> MSEKHPGPLVVEGKLTDAERMKHESNYLRGTIAEDLNDGLTGGFKGDNFLLIRFHGMYQQDDRDIRAERAEQKLEPRHAMLLRCRLPGGVITTKQWQAIDKFAGENTIYGSIRLTNRQTFQFHGILKKNVKPVHQMLHSVGLDALATANDMNRNVLCTSNPYESQLHAEAYEWAKKISEHLLPRTRAYAEIWLDQEKVATTDEEPILGQTYLPRKFKTTVVIPPQNDIDLHANDMNFVAIAENGKLVGFNLLVGGGLSIEHGNKKTYARTASEFGYLPLEHTLAVAEAVVTTQRDWGNRTDRKNAKTKYTLERVGVETFKAEVERRAGIKF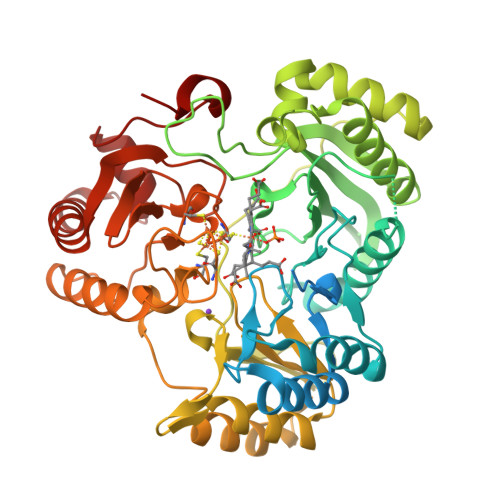EPIRPYEFTGRGDRIGWVKGIDDNWHLTLFIENGRILDYPARPLKTGLLEIAKIHKGDFRITANQNLIIAGVPESEKAKIEKIAKESGLMNAVTPQRENSMACVSFPTCPLAAAEAERFLPSFIDNIDNLMAKHGVSDEHIVMRVTGCPNGCGRAMLAEVGLVGKAPGRYNLHLGGNRIGTRIPRMYKENITEPEILASLDELIGRWAKEREAGEGFGDFTVRAGIIRPVLDPARDLWD> TDMLPEIAAAVGFLSSLLRTRGCVSEQRLKVFSGALQEALTEH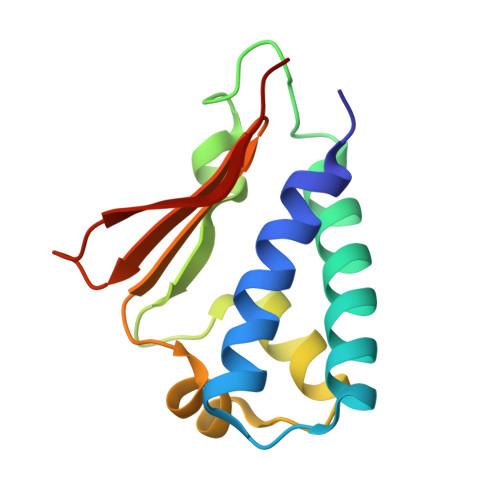YKHHWFPEKPSKGSGYRCIRINHKMDPIISRVASQIGLSQPQLHQLLPSELTLWVDPYEVSYRIGEDGSICVLYEEAPL> MIKNECEKDNQLAARLAKLAGYEKVNGFYKFVNTPEKEMENLGGLLKIVKNLFPDSEEQLLSEYFLELDPNKKCARQSVEYSDINQWDTLTDKIIINLCNSKNSTSQEWGKVYSLHRKLNKNEISLNDAIRESGKCKIKSAEMLFFSNAMLMYAYLNIGEFGLMKSTSKLLEFDDLPEGFIKESFKSRVSMLEANISLNENSLLEARQHSNRAIENSNVNRICFFAYLTIGNTLIFEDYDEAKKAY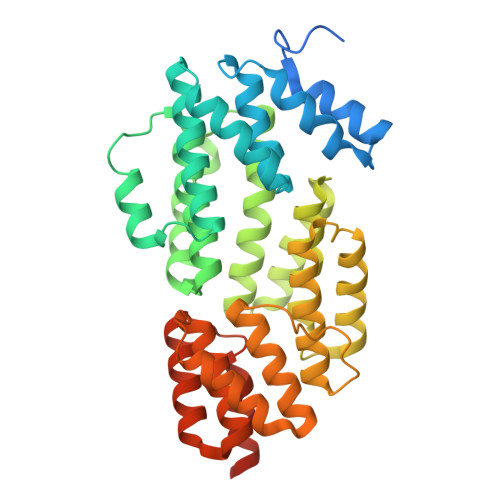IKGQKYAKNPVHQEMLDGALCFLSNIWKKENQWVNYNSDNIKYLQLRAFYYINQGNIEEATEILDELSSRDQDENELGFYYYYKGLISQDKTDYAKSIRYFKKSDDKYFIQLPLLQLERMGADLELLNLISI>[2x]STLRLLISDSYDPWFNLAVEECIFRQMPATQRVLFLWRNADTVVIGRAQNPWKECNTRRMEEDNVRLARRSSGGGAV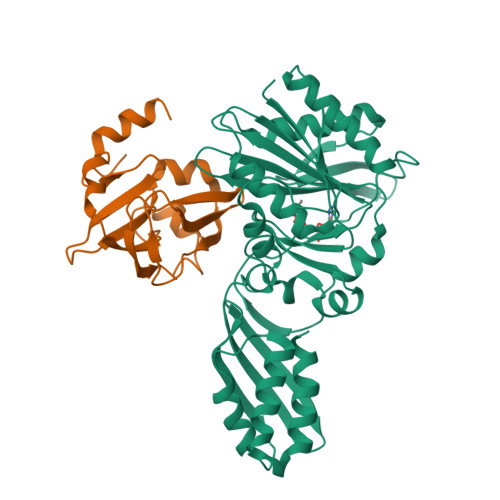FHDLGNTCFTFMAGKPEYDKTISTSIVLNALNALGVSAEASGRNDLVVKTVEGDRKVSGSAYRETKDRGFHHGTLLLNADLSRLANYLNPDKKKLAAKGITSVRSRVTNLTELLPGITHEQVCEAITEAFFAHYGERVEAEIISPNKTPDLPNFAETFARQSSWEWNFGQAPAFSHLLDERFTWGGVELHFDVEKGHITRAQVFTDSLNPAPLEALAGRLQGCLYRADMLQQECEALLVDFPEQEKELRELSAWMAGAVR;>[2x]SNVPAELKYSKEHEWLRKEADGTYTVGITEHAQELLGDMVFVDLPEVGATVSAGDDCAVAESVKAASDIYAPVSGEIVAVNDALSDSPELVNSEPYAGGWIFKIKASDESELESLLDATAYEALLEDE> GSHMSNTQTVLPFTGLNTPSGVAVDSAGTVYVTDRGNNRVVKLAAGSNTQTVLPFTGLNTPSGVAVDSAGTVWVTDHGNNRVVKLAAGSNTQTVLPFTGLNTPSGVAVDSAGTVYVTDRGNNRVVKLAAGSNTQTVLPFTGLNTPSGVAVDSAGTVWVTDHGNNRVVKLAAGSNTQTVLPFTGLNTPSGVAVDSAGTVYVTDRGNN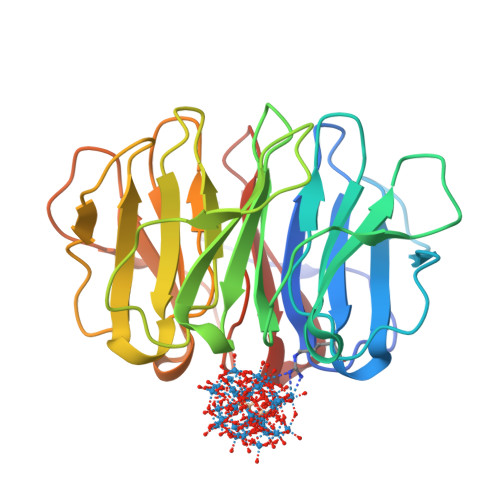RVVKLAAGSNTQTVLPFTGLNTPSGVAVDSAGTVWVTDHGNNRVVKLAAG>[2x]SVYKVLLLGAPGVGKSALARIFGGVEDGPEAEAAGHTYDRSIVVDGE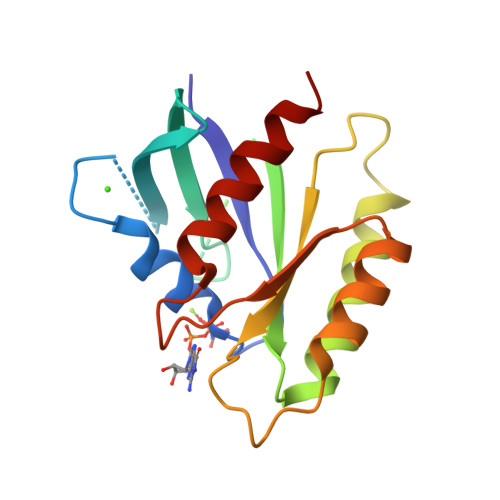EASLMVYDIWEQDGGRWLPGHCMAMGDAYVIVYSVTDKGSFEKASELRVQLRRARQTDDVPIILVGNKSDLVRSREVSVDEGRACAVVFDCKFIETSAALHHNVQALFEGVVRQIRLRR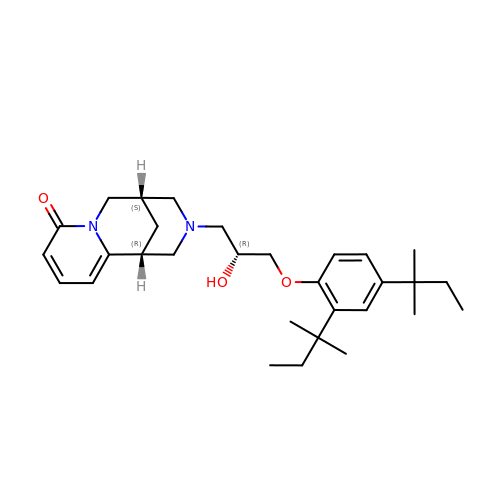(1~{R},9~{S})-11-[(2~{R})-3-[2,4-bis(2-methylbutan-2-yl)phenoxy]-2-oxidanyl-propyl]-7,11-diazatricyclo[7.3.1.0^{2,7}]trideca-2,4-dien-6-one | C30 H44 N2 O3 | ITCUJNFERKWPKY-WMTXJRDZSA-N> MSKNAAVIELGYMGISVKDPDAWKSFATDMLGLQVLDEGEKDRFYLRMDYWHHRIVVHHNGQDDLEYLGWRVAGKPEFEALGQKLIDAGYKIRICD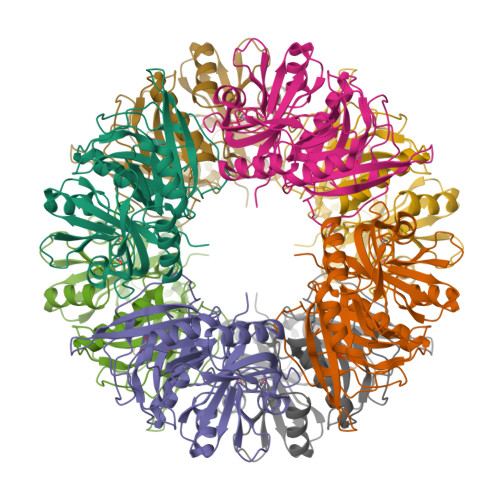KVEAQERMVLGLMKTEDPGGNPTEIFWGPRIDMSNPFHPGRPLHGKFVTGDQGLGHCIVRQTDVAEAHKFYSLLGFRGDVEYRIPLPNGMTAELSFMHCNARDHSIAFGAMPAAKRLNHLMLEYTHMEDLGYTHQQFVKNEIDIALQLGIHANDKALTFYGATPSGWLIEPGWRGATAIDEAEYYVGDIFGHGVEATGYGLDVKLS> GSHMEVNLRMSWWGGNGRHEVTLKALEEFHKEHPNINVKAEYTGWDGHLSRLTTQIAGGTEPDVMQTNWNWLPIFSKDGTGFYNLFSVKEQLDLAQFDPKELQQTTVNGKLNGIPISVTARIFYFNDATWAKAGLEYPKTWDELLAAGQVFKEKLGDQYYPVVLEHQDTLALIRSYMTQKYNIPTIDEANKKFAYSPEQWVEFFTMYKTMVDNHVMPSTKYYASFGKSNMYEMKPWINGEWAGTYMWNSTITKYSDNLTKPAKLVLGPYPMLPGAKDAGLFFKPAQMLSIGKSTKHPQESAMLINFLLNSKEG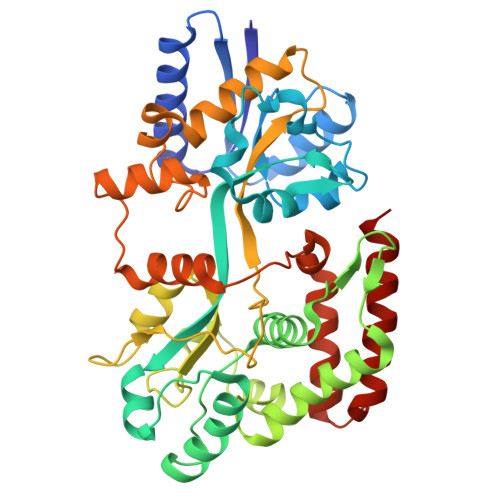VEALGLERGVPLSATAVTQLRASGVIKDEDPSVAGLNMALELPHKMTTSPYFDDPQIVSLFGDAIQYIDYGQKTVQETAEYFNKQGDRILKRAMR>MERNHWNEKSSGAKRSRERDLTLSTIRSILAADERLRIKASSYLGVGRGVDDEAVIDIFPTGQTMSFLRLLHGFLGTCRGQSMHQVLRDPCVLRKQLLYGVCKTLFDTITVRRVAEEWKLHAALFPYRALDEEDLEQYLLVWSASLRQSVQTGVLGALRDILYQYADNDDYGLYVDWCVTVGLVPLLDVKTKPSEAAERAQFVRAAVQRATETHPLAQDLLQANLALLLQVAERLGAVRVANAPEVRVFKKVRSERLEAQLRGKHIRLYVAAEPLAYERDKLLFTTPVAHLHEEILRYDGLCRHQKICQLLNTFPVKVVTASRHELNCKKLVEMMEQHDRGSDAKKSIMKFLLNVSDSKSRIGIEDSVESFLQDLTPSLVDQNRLLPARGPGGPGVVGPGGAVVGGPAGHVGLLPPPPGPAAPERDIRDLFKKQVIKCLEEQIQSQVDEIQDLRTLNQTWENRVRELRDLLTRYASRREDSMSLGARDAELYHLPVLEAVRKARDAAPFRPLAVEDNRLVANSFFSQFVPGTESLERFLTQLWENEYFRTFRLRRLVTHQGAEEAIVYSNYTVERVTLPYLCHILALGTLDPVPEAYLQLSFGEIVAAAYDDSKFCRYVELICSREKARRRQMSREAAGGVPERGTASSGGPGTLERSAPRRLITADEERRGPERVGRFRNGGPDDPRRAGGPYGFH[12x]

Here we present high-resolution structures of the A- and B-capsids and in-situ portals of human cytomegalovirus. The portal proteins are believed to orchestrate nucleation of the procapsid through the formation of a portal–scaffold complex, which facilitates procapsid assembly. During the maturation process, the disassociated scaffold proteins are expelled as the viral DNA is pumped into the capsid through the portal located at a unique vertex of the icosahedral capsid. All three capsids possess a mature icosahedral shell and are distinguishable by the inner capsid material: (1) C-capsids are filled with viral DNA; (2) A-capsids appear empty and are assumed to be products of aborted viral genome packaging; and (3) B-capsids have a featureless inner core consisting of scaffold proteins, likely generated by an unsuccessful initiation of DNA packaging.

Notably, the C12 reconstruction of the B-capsid portal reveals that, among the cluttered scaffold densities surrounding the portal, 12 ordered density fragments tightly encircle the portal crown region. Each of the 12 ordered density fragments has comparable strength to that of the surrounding portal proteins and well matches a 15-residue-long loop-helix-loop motif. More importantly, each of the scaffold fragments is accommodated into a hydrophobic cavity formed by helices from the crown domains of two neighboring pUL104 molecules (helix 110–124 from one molecule and helices 110–124, 134–164, helix-loop-helix 205–225 from another one). Previous biochemical data indicated that tryptophan residues in the portal of HSV-1 are essential to this portal-scaffold interaction. Consistently, we identified two tryptophan residues (Trp118 and Trp142) in the portal that participate in the interaction with the scaffold, and noted that these residues are conserved among herpesviruses. The present study shows that the portal of the B-capsid makes extensive associations with a protruded region of the middle band of the scaffold, which comprises the scaffold domain and 12 loop-helix-loop scaffold fragments that insert into the pockets of the portal crown domain. A portal structural comparison of the DNA-free and DNA-filled capsids shows that the scaffold fragment binding cavity of the portal is closed off in the virion capsid, suggesting that dissociation of the scaffold fragments from the portal is necessary for the required portal conformational changes during DNA translocation. Meanwhile, disengagement of the bound scaffold fragments from the portal would, in turn, release the restraint on the portal to allow for further conformational changes that are required for DNA packaging to proceed.>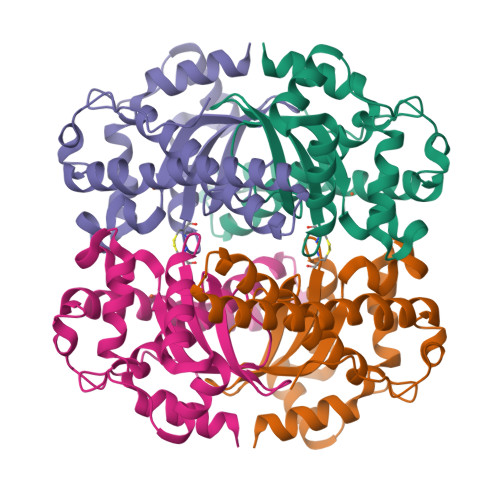[8x]MAEYTLPDLDWDYGALEPHISGQINELHHSKHHATYVKGANDAVAKLEEARAKEDHSAILLNEKNLAFNLAGHVNHTIWWKNLSPNGGDKPTGELAAAIADAFGSFDKFRAQFHAAATTVQGCGWAALGWDTLGNKLLIFQVYDHQTNFPLGIVPLLLLDMWEHAFYLQYKNVKVDFAKAFWNVVNWADVQSRYAAATSQTKGLIFG(2R)-2-[5-(6-amino-5-{(1R)-1-[2-(1,3-dihydro-2H-1,2,3-triazol-2-yl)-5-fluorophenyl]ethoxy}pyridin-3-yl)-4-methyl-1,3-thiazol-2-yl]propane-1,2-diol 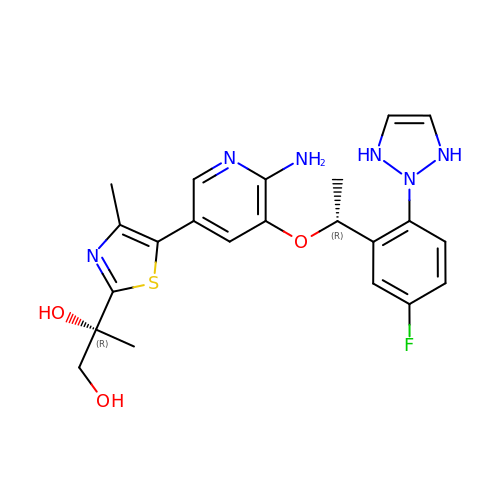| C22 H25 F N6 O3 S | MXETZPYUZKZIMB-MCMMXHMISA-N>[3x]MRRTTKETDIIVEIGKKGEIKTNDLILDHMLTAFAFYLGKDMRITATYDLRHHLWEDIGITLGEALRENLPEKFTRFGNAIMPMDDALVLVSVDISNRPYANVDVNIKDAEEGFAVSLLKEFVWGLARGLRATIHIKQLSGENAHHIVEAAFKGLGMALRVATKESERVESTKGVL

The program of herbicide development described herein aims to identify inhibitors of imidazoleglycerolphosphate‐dehydratase (IGPD; EC 4.2.1.19), an enzyme of histidine biosynthesis in plants and microorganisms. This enzyme catalyzes the manganese(II)‐dependent dehydration of (2R,3S)‐2,3‐dihydroxy‐3‐(1H‐imidazol‐5‐yl)propyl dihydrogen phosphate (2R,3S‐IGP) to 3‐(1H‐Imidazol‐4‐yl)‐2‐oxopropyl dihydrogen phosphate (IAP).4 IGPD shows strict enantioselectivity for its substrate, with the other three diastereoisomers of IGP acting as competitive inhibitors of the enzyme, thus indicating that the active site shows some flexibility to accommodate inverted chiral centers. Previous studies have shown that IGPD is inhibited by triazolylphosphonates, whose potency is based on mimicking key reaction intermediates. In this paper we describe work on the lead compound, 2‐hydroxy‐3‐(1,2,4‐triazol‐1‐yl) propylphosphonate (C348) and present a series of structures of IGPD, from Arabidopsis thaliana, complexed with a synthetic racemate of C348 and with the enantiopure compounds.

Significantly, the mirror‐image packing of the two enantiomers of C348 in IGPD2 gives rise to equipotency and, as in d/l‐AOPP superinhibitors of phenylalanine ammonia‐lyase, the mimicry of a reaction intermediate gives rise to potent inhibition. This study adds to the ever‐growing body of evidence that certain enzymes are chirally promiscuous and that mirror‐image packing of ligands is a more common feature than is generally recognized in the field of drug development.> PPYLKWA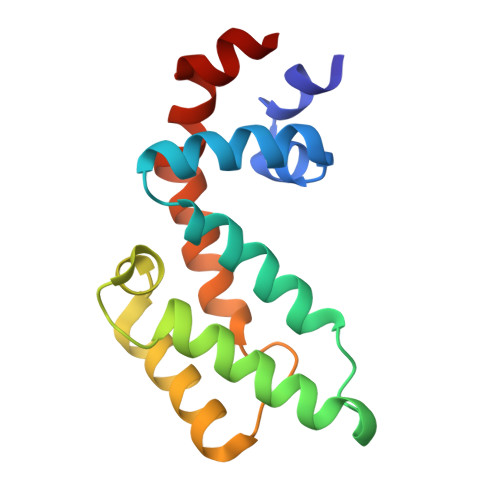ESLHSLLDDQDGISLFRTFLKQEGCADLLDFWFACTGFRKLEPCDSNEEKRLKLARAIYRKYILDNNGIVSRQTKPATKSFIKGCIMKQLIDPAMFDQAQTEIQATMEENTYPSFLKSDIYLEYT>SVKSEYAEAAAVGQEAVAVFNTMKAAFQNGDKEAVAQYLARLASLYTRHEELLNRILEKARREGNKEAVTLMNEFTATFQTGKSIFN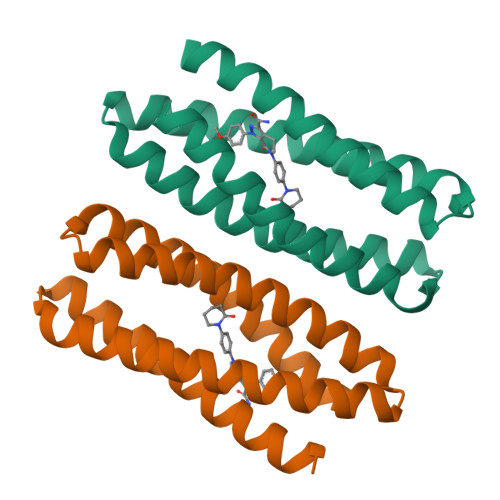AMVAAFKNGDDDSFESYLQALEKVTAKGETLADQIAKAL[2x]>SGHGMEENGMKSKILIFGGTGYIGNHMVKGSLKLGHPTYVFTRPNSSKTTLLDEFQSLGAIIVKGELDEHEKLVELMKKVDVVISALAFPQILDQFKILEAIKVAGNIKRFLPSDFGVEEDRINALPPFEALIERKRMIRRAIEEANIPYTYVSANCFASYFINYLLRPYDPKDEITVYGTGEAKFAMNYEQDIGLYTIKVATDPRALNRVVIYRPSTNIITQLELISRWEKKIGKKFKKIHVPEEEIVALTKELPEPENIPIAILHCLFIDGATMSYDFKENDVEASTLYPELKFTTIDELLDIFVHDPPPPASAAF[2x]

The basil EGS and petunia IGS are closely related to a number of other NADPH-dependent enzymes that act on phenylpropanoid-derived substrates. Structurally, the PIP-family proteins organize around an N-terminal, Rossman-fold domain, containing a core, six-stranded parallel β-sheet flanked on each face by an α-helical layer. In summary, a mechanistic scheme emerges in which binding of the coniferyl acetate substrate within the active site of EGS leads to deprotonation of the p-hydroxy group (PUSH) coupled with expulsion of acetate ion from the C1 substituent (PULL).

The structures of EGS complexed with NADP+ or NADPH provide the first structural characterization of nicotinamide-cofactor binding by the PIP family of enzymes (previous crystallographic analyses had yielded only apo-enzyme structures). Structural differences between the NADP+ and NADPH complexes of EGS are small, and center around the nicotinamide ring of the cofactor. The nicotinamide forms a planar group in the oxidized state, but is distorted slightly to a more boat-like conformation in the reduced state. The nicotinamide ring adopts the anti conformation with its B-face stacked against the side chain of Phe154 and its A-face directed towards the substrate-binding pocket. In contrast, the anti-conformer of the nicotinamide ring observed in EGS is consistent with the class-A reductase (donation of the pro-R hydride) activity of the PIP-family enzymes.>PYVTISATEGLSAEKKKQLLERSSDAVVQSIGAPLASVRVMLHELPGGHYLNAGQFNT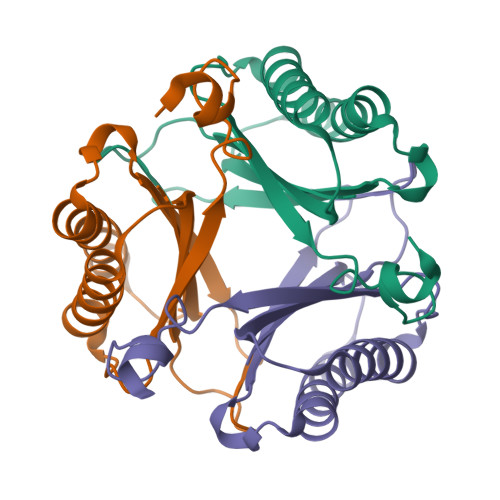PGLMFVVDFIEGRTEEQRNALIAALSKTGTETTGIPESEVRVRLLDFPKANMGMAGGISAKAMGR[6x]> GSDILQELLRVSEKAANIARACRQQETLFQLLIEEKKEGEKNKKFAVDFKTLADVLVQEVIKENMENKFPGLGKKIFGEESNELTNDLGEKIIMRLGPTEEETVALLSKVLNGNKLASEALAKVVHQDVFFSDPALDSVEINIPQDILGIWVDPIDSTYQYIKGSADITPNQGIFPSGLQCVTVLIGVYDIQTGVPLMGVINQPFVSQDL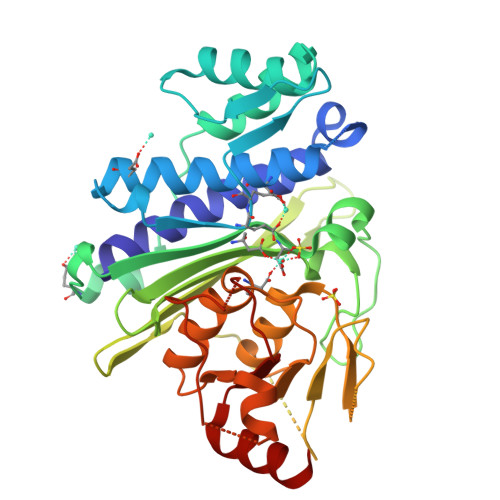HTRRWKGQCYWGLSYLGTNIHSLLPPVSTRSNSEAQSQGTQNPSSEGSCRFSVVISTSEKETIKGALSHVCGERIFRAAGAGYKSLCVILGLADIYIFSEDTTFKWDSCAAHAILRAMGGGMVDLKECLERNPDTGLDLPQLVYHVGNEGAAGVDQWANKGGLIAYRSEKQLETFLSRL HmuTUV forms an ABC-type heme transporter system, in which HmuT, HmuU, and HmuV are the heme binding lipoprotein, permease, and ATPase, respectively. CgHmuT consists of two lobes connected with a α-helix, both of which consist of a five-stranded β-sheet and four α-helices. His141 and Tyr240 are coordinated to the heme as the axial ligands and Arg242 forms a hydrogen bond with Tyr240 in CgHmuT. As CgHmuT is a substrate (heme) binding protein that shuttles heme to the cognate ABC-type heme transporter CgHmuUV in Corynebacteria, the regulation of heme binding and release is very important for its physiological function.

The purified heme-bound proteins were crystallized, and the crystal structures of H141A-, Y240A-, and R242A-CgHmuT were determined in the holo-form at the resolution of 1.30, 1.65, and 1.30 Å, respectively. The distance between the oxygen atom of the OH group in Tyr240 and iron was 2.0 Å, which was identical to that for wild-type CgHmuT. The side chains of Tyr240 and Arg242 were entirely superimposable between wild-type and H141A mutants. On the other hand, the conformation of the loop composed from Gly139 to Ala141 was slightly perturbed by the mutation of His141 to Ala, while other parts were almost superimposable between them. A water molecule was observed at the same position as that of the nitrogen atom of His141 in wild-type CgHmuT. The distance between the water and the iron was 2.6 Å. Though wild-type ferric CgHmuT is not reduced by dithionite, probably due to a low redox potential of the heme, H141A-CgHmuT was reduced by dithionite. The ν2 and ν3 bands at 1583 and 1487 cm−1, respectively, are due to a five-coordinate high spin heme, while those at 1571 and 1480 cm−1 are due to a six-coordinate high spin heme. The equilibrium will be present in the H141A-CgHmuT solution for the coordination/dissociation of water to/from the heme iron.

> MASWDSPTASSNGDLIEEIQASSTSTDPRTFTGLSIVEDIGDVVPVTDNASPALPVSLTDADGNDVVVEDVSRILPLDLYGTYSKTIAGLGLVDNIVGRTVSSTEPALADTEVVTTGGATLNAEAILNLHPTLVIIDHSIGPREVIDQIRAAGVATVIMSPQRSIASIGDDIRDIASVVGLPEEGEKLAERSVAEVEEASTVVDELTPEDPLKMVFLYARGTGGVFFILGDAYGGRDLIEGLGGVDMAAEKGIMDLAPANAEALAELNPDVFVMMSEGLVSTGGIDGLMERPGIAQTTAGQNQRVLALPDGQSLAFGAQTGELLLRASRELYVQGGELEHHHHHH>[2x]MMASAATELDVDGVKV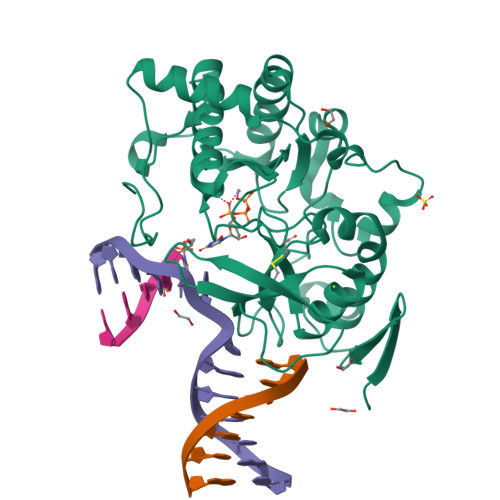RFTNPDKVYFPKLGKNGTKGKLVEYYLSVASGPMLALLRDRPVHLQRFPDGIEGEEIYQKRVPQKHPDYLETCVVTFPSGRTADALKITHPSSIIWAAQMGTVTLHPWQVRCPDTEHPDELRVDLDPQPGTGFKEARTVACDVLKPLLDELGLVGYPKTSGGRGVHVFLRIKPQWDFIEVRRAGIALAREVERRAPDAVTTSWWKEERGERLFIDYNQNARDRTFASAYSVRKTPIATVSMPLSWDELRNADPDDYTMNTVPDLLAGRDDPWADIDSVQQSLGPLLDLVAADEERGLGDLPYPPNYPKMPGEPPRVQPSKKVAEHWDEQGNRKQ> MGSSHHHHHHSQDLMVTSTYIPMSQRRSWADVKPIMQDDGPNPVVPIMYSEEYKDAMDYFRAIAAKEEKSERALELTEIIVRMNPAHYTVWQYRFSLLTSLNKSLEDELRLMNEFAVQNLKSYQVWHHRLLLLDRISPQDPVSEIEYIHGSLLPDPKNYHTWAYLHWLYSHFSTLGRISEAQWGSELDWCNEMLRVDGRNNSAWGWRWYLRVSR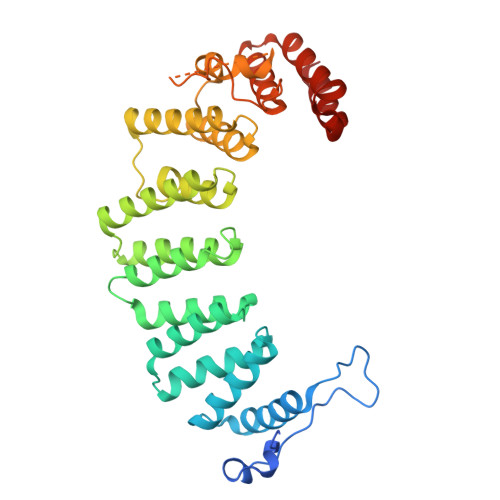PGAETSSRSLQDELIYILKSIHLIPHNVSAWNYLRGFLKHFSLPLVPILPAILPYTASKLNPDIETVEAFGFPMPSDPLPEDTPLPVPLALEYLADSFIEQNRVDDAAKVFEKLSSEYDQMRAGYWEFRRRECAE> MSPKSPVASASAFESVEESDDDDNLTNSEGLDASYLQANGDNEMPADANEEQISMAASSMIRSHSVSGDLHGVQPDPIAADILRKEPEQETFVRLNVPLEVPTSDEVEAYKCLQECLELRKRYVFQETVAPWEKEVISDPSTPKPNTEPFAHYPQGKSDHCFEMQDGVVHVFANKDAKEDLFPVADATAFFTDLHHVLKVIAAGNIRTLCHRRLVLLEQKFNLHLMLNADKEFLAQKSAPHRDFYNVRKVDTHVHHSACMNQKHLLRFIKSKLRKEPDEVVIFRDGTYLTLREVFESLDLTGYDLNVDLLDVHADKSTFHRFDKFNLKYNPCGQS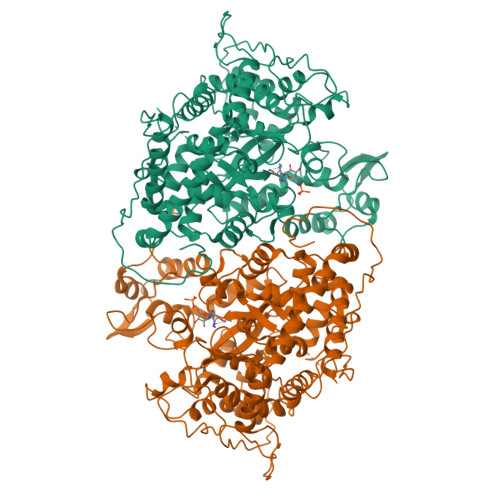RLREIFLKQDNLIQGRFLGEITKQVFSDLEASKYQMAEYRISIYGRKMSEWDQLASWIVNNDLYSENVVWLIQLPRLYNIYKDMGIVTSFQNILDNIFIPLFEATVDPDSHPQLHVFLKQVVGFDLVDDESKPERRPTKHMPTPAQWTNAFNPAFSYYVYYCYANLYVLNKLRESKGMTTITLRPHSGEAGDIDHLAATFLTCHSIAHGINLRKSPVLQYLYYLAQIGLAMSPLSNNSLFLDYHRNPFPVFFLRGLNVSLSTDDPLQIHLTKEPLVEEYSIAASVWKLSACDLCEIARNSVYQSGFSHALKSHWIGKDYYKRGPDGNDIHKTNVPHIRVEFRDTIWKEEMQQVYLGKAVISDEVVP methyl 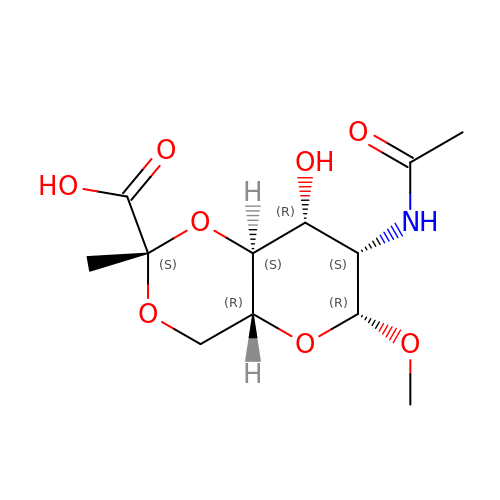2-(acetylamino)-4,6-O-[(1S)-1-carboxyethylidene]-2-deoxy-beta-D-mannopyranoside | C12 H19 N O8 | KCXDWSUMIHDAQQ-KFRVFMFJSA-N>[4x]AQSVPPGDIQTQPGTKIVFNAPYDDKHTYHIKVINSSARRIGYGIKTTN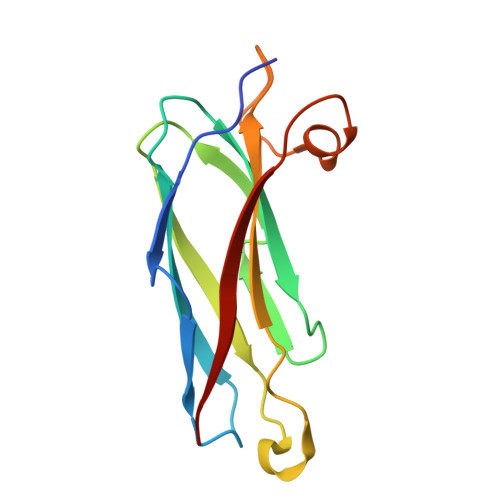MKRLGVDPPCGVLDPKEAVLLAVSCDAFAFGQEDTNNDRITVEWTNTPDGAAKQFRREWFQGDGMVRRKNLPIEYNP>[2x]SNAMLTPISIEKEHIRLINLLHFINEQNRWFTIKELSDYLQVADKTVRKYLKLLEDEIPPSW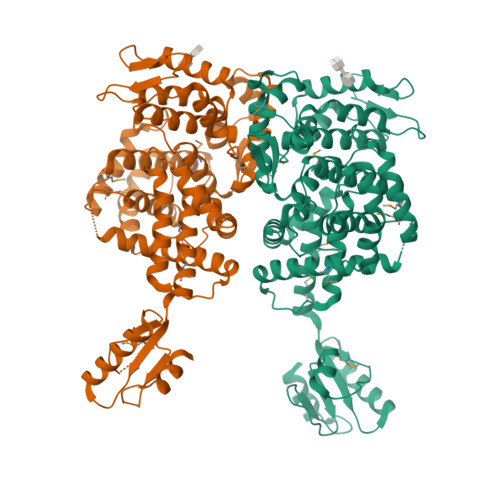NLLVQKGKGIYLKKPLNESLSFVESKILRKSLNLQICEELVFKKNSMQSLAQKLHLQVGALYPIINQINYDIQSSHLNIKKKPLEISGREQDVRVFMLRLYCNIPNDYWPFPYINKQNITDLINKMEKILNVQMYTYSKHKLCVLFAITISRLLSGNTIDNVSGLILVNKNDDHYKTVASITSELQNSFGVTLHETEISFLALALLLSLGNSITTDSNKTLTSYKKTIMPLAKEITKGIEHKLQLGINYDESFLTYVVLIIKKALDKNFIQYYNYNIKFIRHIKQRHPNTFNTIQECISNLNYTVYSHFDCYEISLLTMHFETQRMLFKNNPKKIYVYTSQGCIHREYISALLEKRYNGLIKIVRNTIINLTNESLQDMEIDIIISNVNLPIKNIPIVQISEFPTERDFHEIKKII> 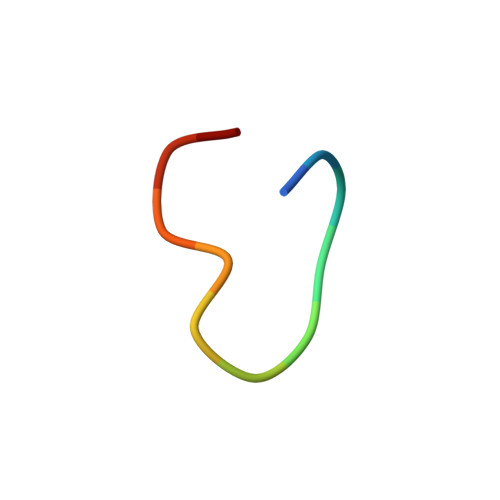CWWKKKKKWWCX> GILANLKEPSAHWCRKMRTVFRPWDVEGGSKGYVTE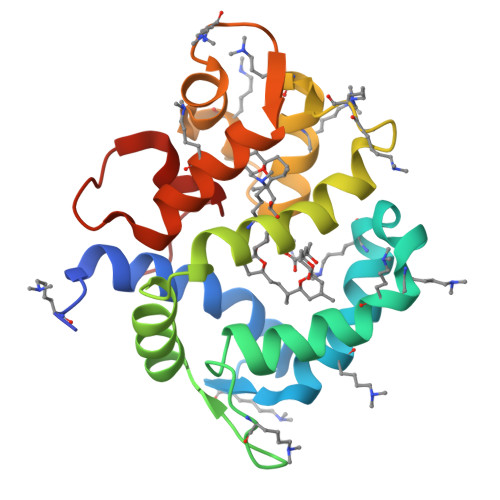EVFKDGVQRRLEKFPELAPTKDKMYERSHRHWVNHCNLGVKMPEGYRLTESQYVQNAWLLIHSPDFEASLKESSQTFWEGIDREKKGYITKEEATKLGIRVTKDPNLKSTGIFEAMDEKNTGRITFEDTLKAQLFFFTDQDNTTHPFNYVRGALVD> FSTPVDIDIVLADADKRAMVDVKLDKNRREKVPLYMDGESVKGCVTVRPKDGKRLEHT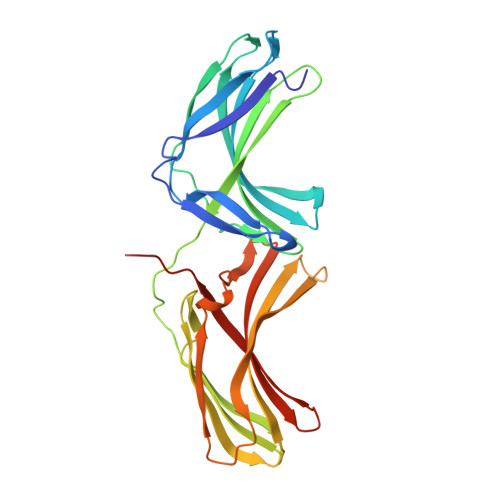GIKVQFIGTIEMFFDRGNHYEFLSLVQELAAPGELQHPQTFDFNFKNVEKQYESYNGINVKLRYFVRVTVSRRMADVIREKDIWVYSYRIPPELNSSIKMDVGIEDCLHIEFEYSKSKYHLKDVIVGRIYFLLVRLKIKHMELSIIRRETTGVAPNQYNESETLVRFEIMDGSPSRGETIPIRLFLGGFDLTPTFRDVNKKFSTRYYLSLVLIDEDARRYFKQSEIILYRQPPE> GPLGSMSSIGLAHNVTILGSGETTVVLGHGYGTDQSVWKLLVPYLVDDYKVLLYDHMGAGTTNPDYFDFDRYSSLEGYSYDLIAILEEFQVSKCIYVG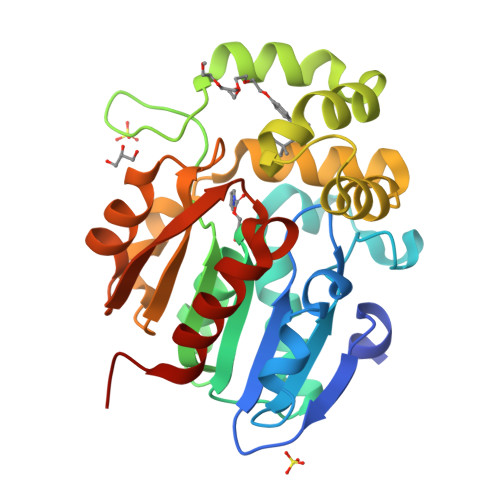HSMSSMAAAVASIFRPDLFHKLVMISPTPRLINTEEYYGGFEQKVMDETLRSLDENFKSLSLGTAPLLLACDLESAAMQEYCRTLFNMRPDIACCITRMICGLDLRPYLGHVTVPCHIIQSSNDIMVPVAVGEYLRKNLGGPSVVEVMPTEGHLPHLSMPEVTIPVVLRHIRQDITDH> LSKVVIRRLPPTLTKEQLQEHLQPMPEHDYFEFFS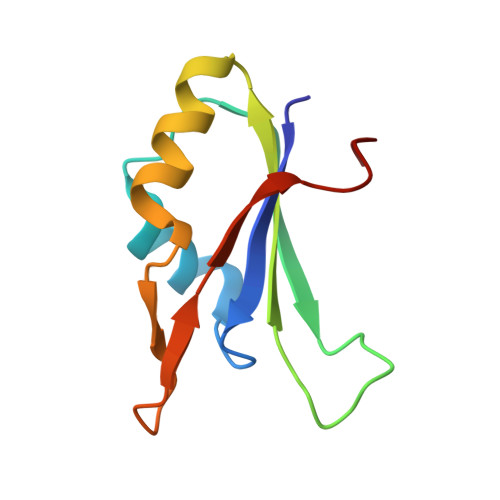NDTSLYPHMYARAYINFKNQEDIILFRDRFDGYVFLDNKGQEYPAIVEFAPFQKAA> MAQPSTTYKFELNLTDLDRGVYESVKQTIARHPSETEERMTVRLLAYAFWYNEQLAFGRGLSDVDEPALWEKSLDDRVLHWIEVGQPDADRLTWCSRRTERTSLLAYGSLRVWEGKVIPAIKNLKNVNIAAVPQDVLEVLAKDMPR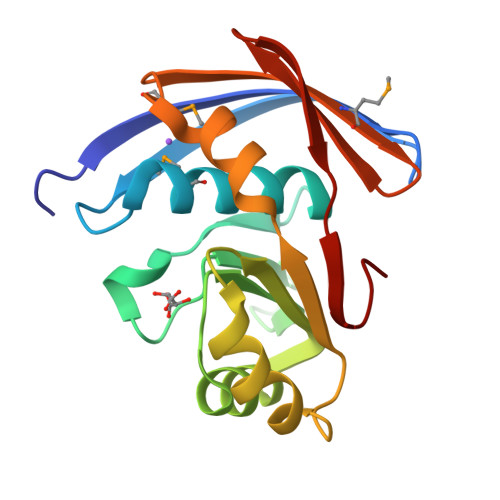VIKWDVMISEGTVFVTDDRGQHEVQLQWLTGERG>[2x]HTIF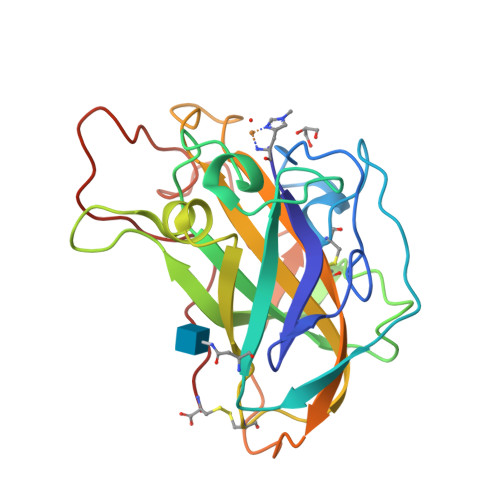SSLEVNGVNQGLGEGVRVPTYNGPIEDVTSASIACNGSPNTVASTSKVITVQAGTNVTAIWRYMLSTTGDSPADVMDSSHKGPTIAYLKKVDNAATASGVGNGWFKIQQDGMDSSGVWGTERVINGKGRHSIKIPECIAPGQYLLRAEMIALHAASNYPGAQFYMECAQLNVVGGTGAKTPSTVSFPGAYSGSDPGVKISIYWPPVTAYTVPGPSVFTC N-(3-chlorophenyl)-2-phenylacetamide | C14 H12 Cl N O | 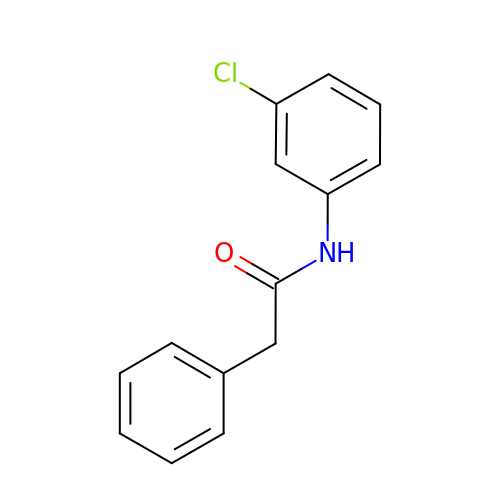GAWITMMQHFGOMV-UHFFFAOYSA-N>[3x]TSELRICRINKESGPCTGGEELY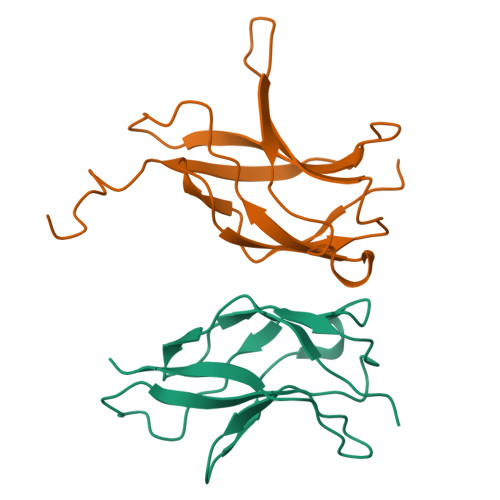LLCDKVQKEDISVVFSTASWEGRADFSQADVHRQIAIVFKTPPYEDLEISEPVTVNVFLQRLTDGVCSEPLPFTYLPR;>[3x]ASNLKIVRMDRTAGCVTGGEEIYLLCDKVQKDDIQIRFYEEEENGGVWEGFGDFSPTDVHRQFAIVFKTPKYKDVNITKPASVFVQLRRKSDLETSEPKPFLYYPEIKDKEEVQR> TTDTRRRVKLYALNAERQWDDRGTGHVSSTYVERLKGISLLVRAESDGSLLLESKIQPDTAYQKQQDTLIVWSEGDNFDLALSFQEKAGCDEIWEKICQVQGKDPSVEITQDIVEESEDERF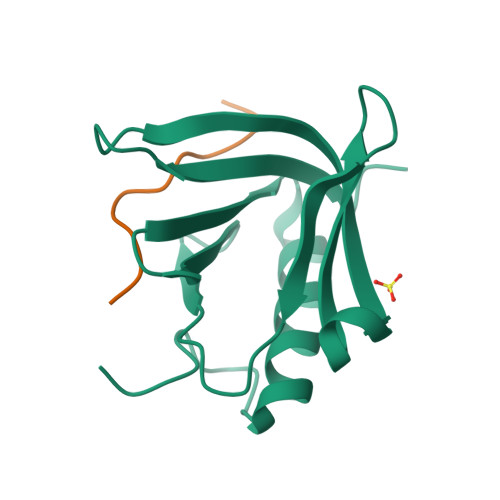;> PDESSADVVFKKPLAPAPR> MGSHHHHHHGSENLYFQSAKDERAREILRGFKLNWMNLRDAETGKILWQGTEDLSVPGVEHEARVPKKILKCKAVS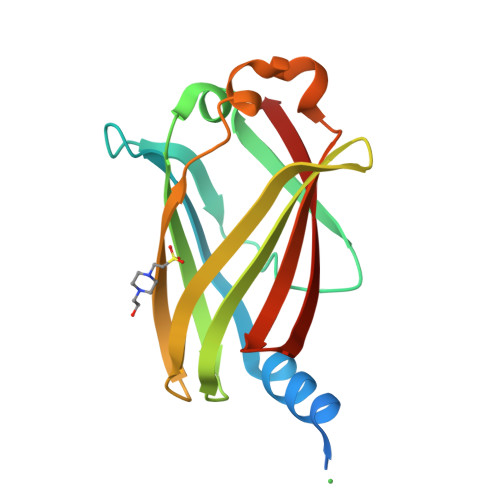RELNFSSTEQMEKFRLEQKVYFKGQCLEEWFFEFGFVIPNSTNTWQSLIEAAPESQMMPASVLTGNVIIETKFFDDDLLVSTSRVRLFYV>[3x]MSSLDINEQRALIKSAHRYISEKLEDHFSSEFLPKALVICGSGLSGISTKIADEPKPLILSYSTIPGFKVSTVP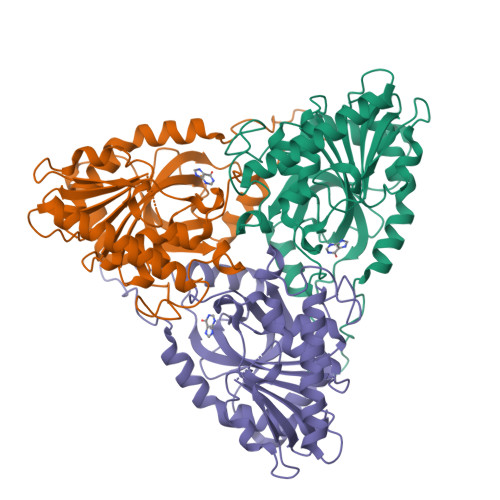GHSGELIFGYMNGAPVVLMNGRLHSYEGHSLAETVHPIRALHLLGSINVLIVTNAAGGINASFKAGDLMCVYDHINFPGLCGFHPLRGANFDEFGPRFLATSDAYDLELRKLLFSKKKELNIERKIHEGTYSYVHGPTFESRAESRFLRLAGTDAVGMSTVPEVVTARHCGWRVLALSLITNECVVDPPASAHDENPVPIQEGKATHEEVLENSAKASKDVQELIFSVVAEIHHHHHH N-acetyl glucosamine-binding protein A (GbpA) is an adhesin that binds to the chitinaceous surface of zooplankton and breaks its dense crystalline packing thanks to its lytic polysaccharide monooxygenase (LPMO) activity, which provides V. cholerae with nutrients. In addition, GbpA is an important colonization factor associated with bacterial pathogenicity, allowing the binding to mucins in the host intestine. The oxidative activity of LPMOs depends on a copper ion bound by a histidine brace motif. Here, we report the discovery of a cation-binding site in proximity of the GbpA active site, which allows Ca2+, Mg2+, or K+ binding close to its carbohydrate-binding surface.

The crystal structures of the LPMO-calcium and LPMO-potassium complexes were refined to 1.8 Å and 1.5 Å, respectively, with R/R free values of 0.179/0.228 and 0.164/0.192. In both structures, a cation-binding site was identified close to the copper-binding active site of the LPMO. The cation-binding site is formed mainly by the loop located between strands 7 and 8 of the core β-sandwich characteristic of LPMOs. This includes the backbone carbonyl groups of Val186, Thr189, and Ala191 as well as the side chain carboxylate of Asp185. In addition, coordination by the side chain carboxylate of Asp70, located in the L2 region, is key to binding. The coordination geometry for K+ is that of a tetragonal bipyramid, that is, octahedral, whereas Ca2+ coordination is characterized by a distorted pentagonal bipyramid, with the two carboxyl oxygens of Asp70 involved in the interaction. In contrast, monovalent cations appear to confer only small stabilizing or destabilizing effects on GbpA, with equivalent trends observed for Na+ and K+. The role of K+ remains enigmatic. In terms of protein stability, the presence of a potassium ion in the metal-binding site might be equivalent to that of the lysine residue from loop L2, which occupies the metal-binding site in some AA10 LPMOs.

>[2x]HGYVSAVENGVAEGRVTLCKFAANGTGEKNTHCGAIQYEPQSVEGPDGFPVTGPRDGKIASAESALAAALDEQTADRWVKRPIQAGPQTFEWTFTANHVTKDWKYYITKPNWNPNQPLSRDAFDLNPFCVVEGNMVQPPKRVSHECIVPEREGYQVILAVWDVGDTAASFYNVIDVKFDG>MEIAFLLNGETRRVRIEDPTQSLLELLRAEGLTGTKEGCNEGDCGACTVMIRDAAGSRAVNACLMMLPQIAGKALRTIEGIAAPDGRLHPVQQAMIDHHGSQCGFCTPGFIVSMAAAHDRDRKDYDDLLAGNLCRCTGYAPILRAAEAAAGEPPADWLQADAAFTLAQLSSGVRGQTAPAFLPETSDALADWYLAHPEATLIAGGTDVSLWVTKALRDLPEVAFLSHCKDLAQIRETPDGYGIGAGVTIAALRAFAEGPHPALAGLLRRFASEQVRQVATIGGNIANGSPIGDGPPALIAMGASLTLRRGQERRRMPLEDFFLEYRKQDRRPGEFVESVTLPKSAPGLRCYKLSKRFDQDISAVCGCLNLTLKGSKIETARIAFGGMAGVPKRAAAFEAALIGQDFREDTIAAALPLLAQDFTPLSDMRASAAYRMNAAQAMALRYVRELSGEAVAVLEVMP[4x];>MSVGKPLPHDSARAHVTGQARYLDDLPCPANTLHLAFGLSTEASAAITGLDLEPVRESPGVIAVFTAADLPHDNDASPAPSPEPVLATGEVHFVGQPIFLVAATSHRAARIAARKARITYAPRPAILTLDQALAADSRFEGGPVIWARGDVETALAGAAHLAEGCFEIGGQEHFYLEGQAALALPAEGGVVIHCSSQHPSEIQHKVAHALGLAFHDVRVEMRRMGGGFGGKESQGNHLAIACAVAARATGRPCKMRYDRDDDMVITGKRHDFRIRYRIGADASGKLLGADFVHLARCGWSADLSLPVCDRAMLHADGSYFVPALRIESHRLRTNTQSNTAFRGFGGPQGALGMERAIEHLARGMGRDPAELRALNFYDPPERGGLSAPPSPPEPIATKKTQTTHYGQEVADCVLGELVTRLQKSANFTTRRAEIAAWNSTNRTLARGIALSPVKFGISFTLTHLNQAGALVQIYTDGSVALNHGGTEMGQGLHAKMVQVAAAVLGIDPVQVRITATDTSKVPNTSATAASSGADMNGMAVKDACETLRGRLAGFVAAREGCAARDVIFDAGQVQASGKSWRFAEIVAAAYMARISLSATGFYATPKLSWDRLRGQGRPFLYFAYGAAITEVVIDRLTGEN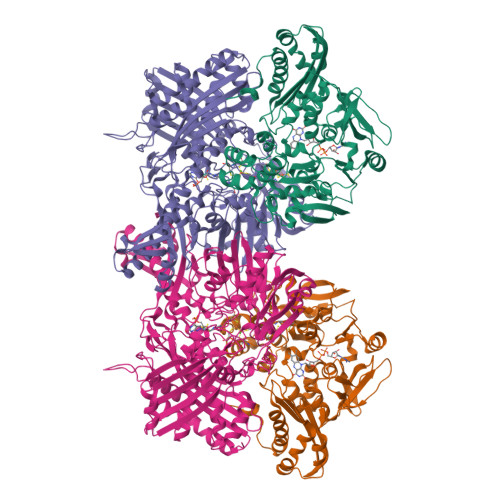RILRTDILHDAGASLNPALDIGQIEGAYVQGAGWLTTEELVWDHCGRLMTHAPSTYKIPAFSDRPRIFNVALWDQPNREETIFRSKAVGEPPFLLGISAFLALHDACAACGPHWPDLQAPATPEAVLAAVRRAEGRA[4x]> GKPEAQPFAHLTINAASIPSGSHKVTLSSWYHDRGWAKISNMTLSNGKLRVNQDGFYYLYA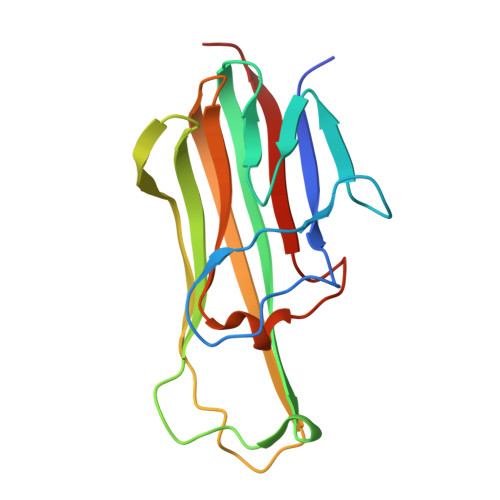NICFRHHETSGSVPTDYLQLMVYVVKTSIKIPSSHNLMKGGSTKNWSGNSEFHFYSINVGGFFKLRAGEEISIQVSNPSLLDPDQDATYFGAFKVQDID>MGSDKIHHHHHHENLYFQGMELVFDKDGLSAYLEEVFPQIQGEFSIDALAKGEITMRLNVQERHLRPGGTVSGPSMFALADVSVY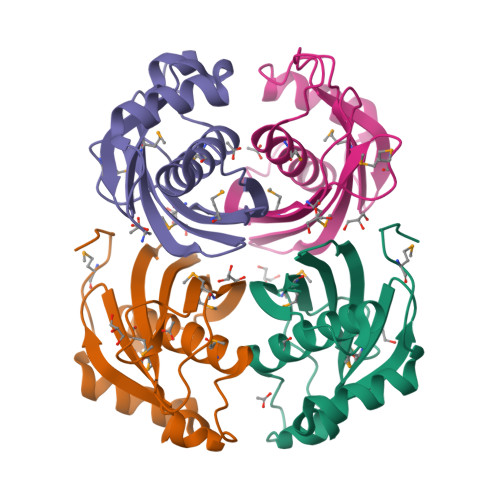ALVLAHLGREALAVTTNASLDFMRKPESGRDLLGQARLLKLGRTLAVGDILLFSEGMEAPVARSTMTYSIPPKR[4x]>[2x]MPKEYGADSITILEGLEAVRKRPGMYIGSTGERGLHHLIWEVVDNAVDEAMAGFATRVDVKIHADGSVEVRDDGRGIPVEMHATGMPTIDVVMTQVGVSVVNALSTRLEATVLRDGYEWF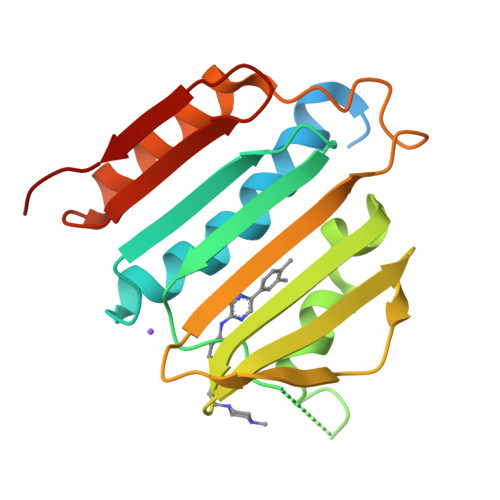QYYDRSVPGKLKQGGETKETGTTIRFWADPEIFETTDYNFETVARRLQEMAFLNKGLTIELTDERDGKHRVFHYPG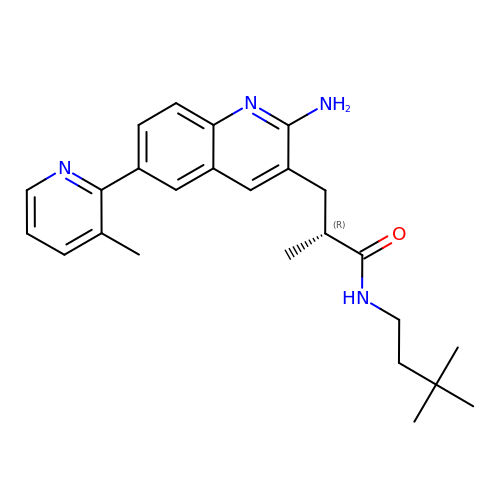(2R)-3-[2-amino-6-(3-methylpyridin-2-yl)quinolin-3-yl]-N-(3,3-dimethylbutyl)-2-methylpropanamide | C25 H32 N4 O | ZVOWIRUWKAUSAB-QGZVFWFLSA-N> MTTSKERHSVSKRLQQELRTLLMSGDPGITAFPDGDNLFKWVA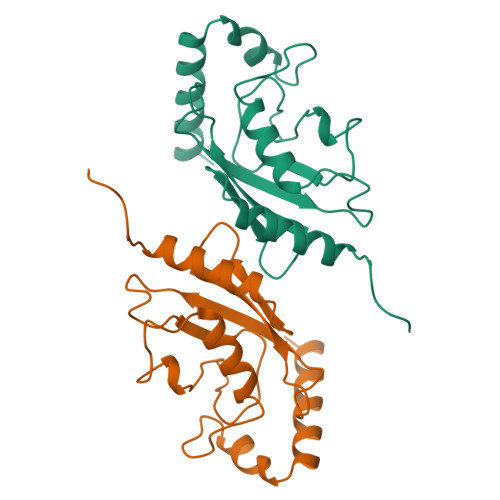TLDGPKDTVYESLKYKLTLEFPSDYPYKPPVVKFTTPCWHPNVDQSGNICLDILKENWTASYDVRTILLSLQSLLGEPNNASPLNAQAADMWSNQTEYKKVLHEKYKTAQSDK>MAAGIVASRRLRDLLTRRLTGSNYPGLSISLRLTGSSAQEEASGVALGEAPDHSYESLRVTSAQKHVLHVQLNRPNKRNAMNKVFWREMVECFNKISRDADCRAVVISGAGKMFTAGIDLMDMASDILQPKGDDVARISWYLRDIITRYQETFNVIERCPKPVIAAVHGGCIGGGVDLVTACDIRYCAQDAFFQVKEVDVGLAADVGTLQRLPKVIGNQSLVNELAFTARKMMADEALGSGLVSRVFPDKEVMLDAALALAAEISSKSPVAVQSTKVNLLYSRDHSVAESLNYVASWNMSMLQTQDLVKSVQATTENKELKT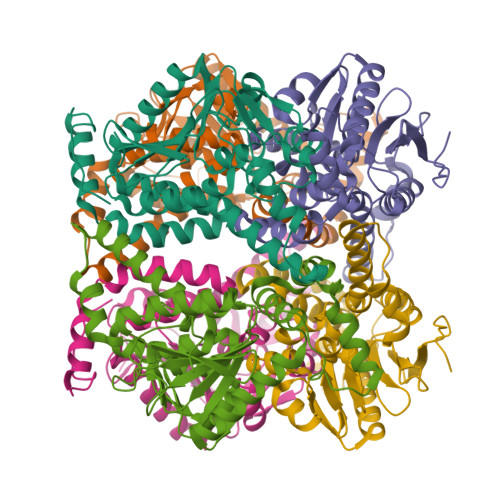VTFSKL[6x]> GMTTENTTALLLIDFQNDYFSTYNGAKNPLV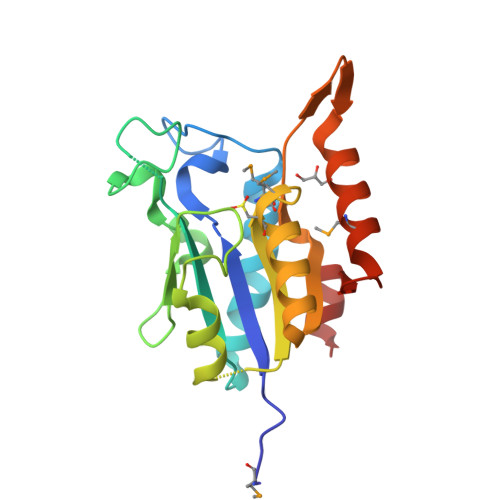GTEAAAEQGAKLLAKFRQQGLPVVHVRHEFPTDEAPFFLPGSDGAKIHPSVAAQEGEAVVLKHQINSFRDTDLKKVLDDAGIKKLVIVGAMTHMCIDAVTRAAEDLGYECAVAHDACATLDLEFNGITVPAAQVHAAFMSALSFAYANVASADELIAGL> S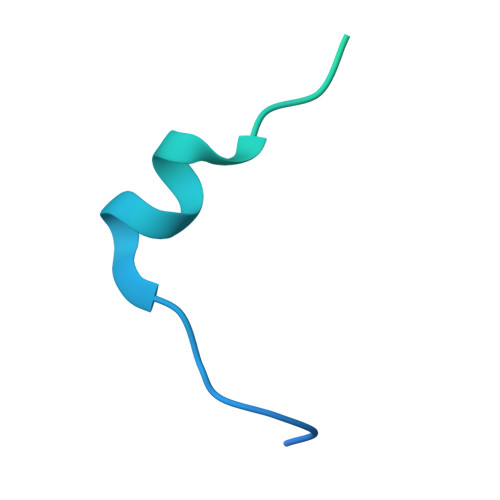NAMSEAKKLNIGRELTDEELMEMTGGSTFSIQCQKDYTYKPSLPVVKYGVVIDEPEVVIKYGVGPIVGIKYGVEPIGPIQPMYGIKPVETLK(6~{R})-6-azanyl-3-nitro-6-oxidanyl-cyclohexa-1,3-diene-1-carboxylic 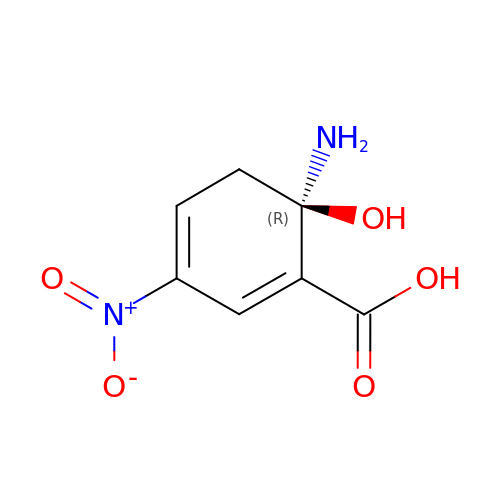acid | C7 H8 N2 O5 | YMJMMSMKJXYRPV-SSDOTTSWSA-N>[2x]MSFMDQIPGGGNYPKLPVECLPNFPIQPSLTFRGRNDSHKLKNFISEIMLNMSMISWPNDASRIVYCRRHLLNPAAQWANDFVQEQGILEITFDTFIQGLYQHFYKPPDINKIFNAITQLSEAKLGIERLNQRFRKIWDRMPPDFMTEKAAIMTYT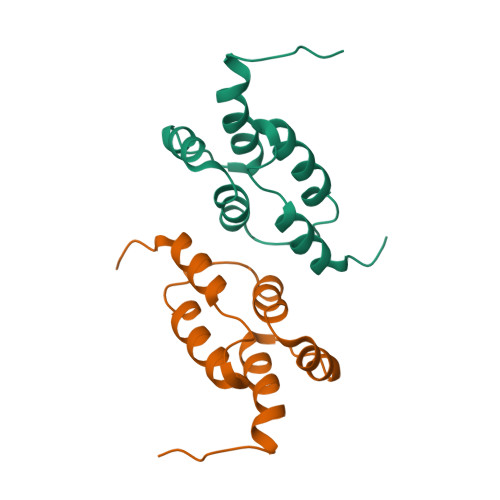RLLTKETYNIVRMHKPETLKDAMEEAYQTTALTERFFPGFELDADGDTIIGATTHLQEEYDSDYDSEDNLTQNRYVHTVRTRRSYNKPMSNHRNRRNNNASREECIKNRLCFYCKKEGHRLNECRARKAVLTDLELESKDQQTLFIKTLPIVH>[12x]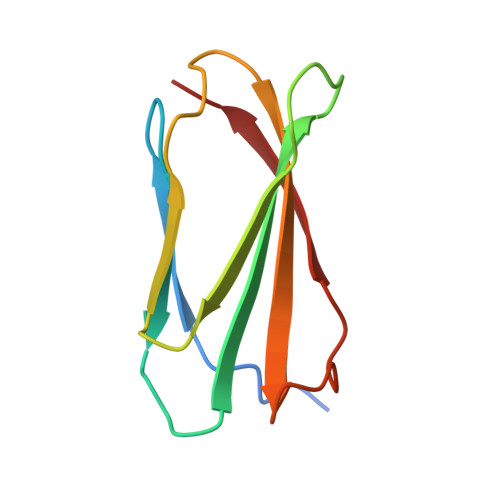GSGLQPGSSIPPYNTEVTETTIVITWTPAPRIGFKLGVRPSQGGEAPREVTSDSGSIVVSGLTPGVEYVYTIQVLRDGQERDAPIVNKVVTP5'-O-[(3-methyl-D-valyl)sulfamoyl]adenosine | C16 H25 N7 O7 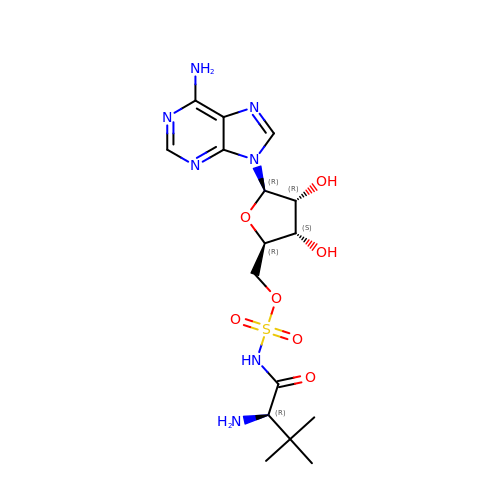S | ZUUYOZYPJCVYHV-YEFHITBRSA-N>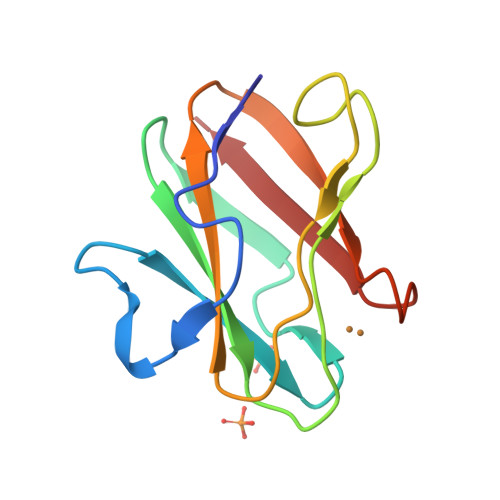 DKATIPSESPFAAAEVADGAIVVDIAKMKYETPELHVKVGDTVTWINREAMPHNVHFVAGVLGEAALKGPMMKKEQAYSLTFTEAGTYDYHCTAHPFMRGKVVVE>[2x]MSCYIYWDKIKRIASRLEGMNYHFDEMDTSGVMPLLDEIEEIAHDSTIDFESAKHILDDAEMNHALSLIRKFYVNLGMKLEMEKAQEVIESDSPWETLRSFYFYPRYLELLKNEAALGRFRRGERAVFIGGGPLPLTGILLSHVYGMRVNVVEIEPDIAELSRKVIEG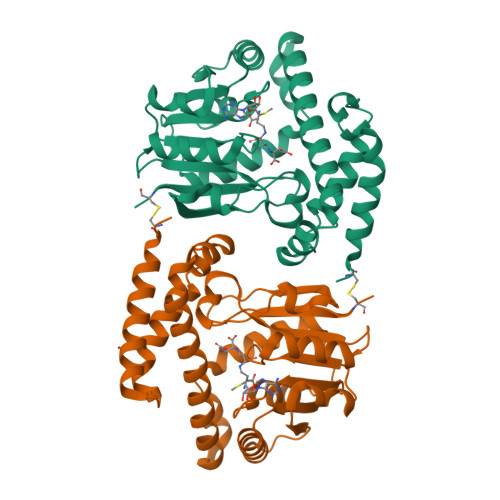LGVDGVNVITGDETVIDGLEFDVLMVAALAEPKRRVFRNIHRYVDTETRIIYRTYTGMRAILYAPVSDDDITGFRRAGVVLPSGKVNNTSVLVFKCPDKGELNSKLEGKPIPNPLLGLDSTRTGHHHHHH N~1~-[(4-fluorophenyl)methyl]-N~1~-methyl-N~4~-(4-methyl-1,3-thiazol-2-yl)piperidine-1,4-dicarboxamide 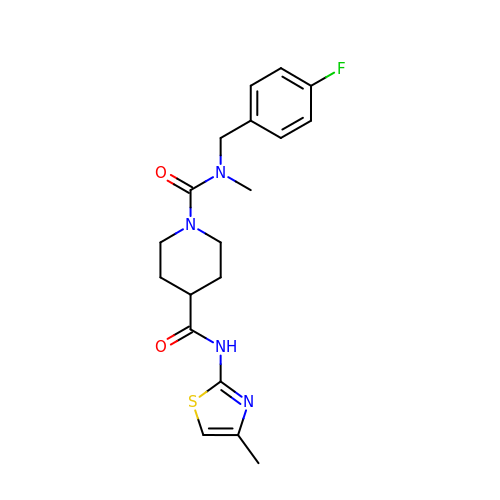| C19 H23 F N4 O2 S | FYQIXROHNRZVMM-UHFFFAOYSA-N>[6x]MRLELPVIPLRNTVILPHTTTPVDVGRAKSKRAVEEAMGADRLIFLVAQRDPEVDDPAPDDLYTWGVQAVVKQAMRLPDGTLQVMVEARARAQVTDYIPGPYLRARGEVFSEIFPIDEAVVRVLVEELKEAFEKY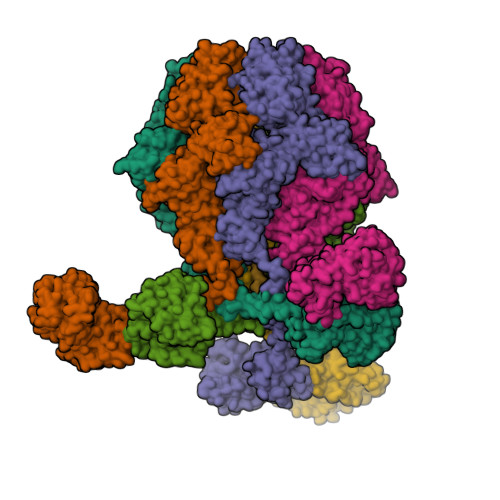VANHKSLRLDRYQLEAVKGTSDPAMLADTIAYHATWTVAEKQEILELTDLEARLKKVLGLLSRDLERFELDKRVAQRVKEQMDTNQREYYLREQMKAIQKELGGEDGLSDLEALRKKIEEVGMPEAVKTKALKELDRLERMQQGSPEATVARTYLDWLTEVPWSKADPEVLDINHTRQVLDEDHYGLKDVKERILEYLAVRQLTQGLDVRNKAPILVLVGPPGVGKTSLGRSIARSMNRKFHRISLGGVRDEAEIRGHRRTYIGAMPGKLIHAMKQVGVINPVILLDEIDKMSSDWRGDPASAMLEVLDPEQNNTFTDHYLDVPYDLSKVFFITTANTLQTIPRPLLDRMEVIEIPGYTNMEKQAIARQYLWPKQVRESGMEGRIEVTDAAILRVISEYTREAGVRGLERELGKIARKGAKFWLEGAWEGLRTIDASDIPTYLGIPRYRPDKAETEPQVGTAQGLAWTPVGGTLLTIEVAAVPGSGKLSLTGQLGEVMKESAQAALTYLRAHTQDYGLPEDFYNKVDLHVHVPDGATPKDGPSAGITMATAIASALSRRPARMDIAMTGEVSLRGKVMPIGGVKEKLLAAHQAGIHKIVLPKDNEAQLEELPKEVLEGLEIKLVEDVGEVLEYLLLPEPTMPPVVQPSDNRQQPGAGA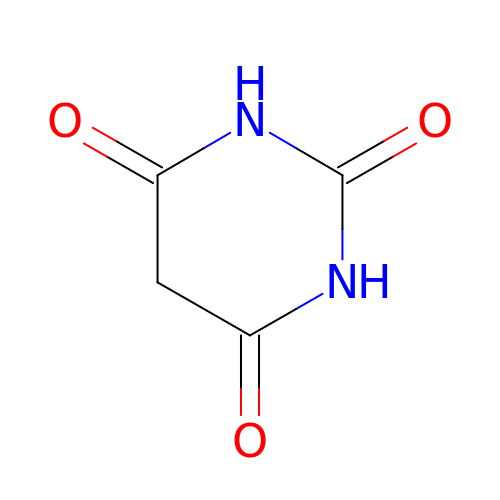BARBITURIC ACID | C4 H4 N2 O3 | HNYOPLTXPVRDBG-UHFFFAOYSA-N> GS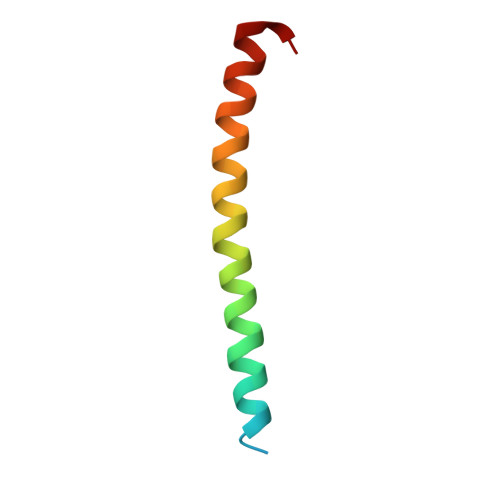KDPDAAKKEEERQEALRQAEEERKAKYAKMEAEREVMRQGIRDKYGI> GSHMQDPEQLKHCNGILKELLSKKHAAYAWPFYKPVDASALGLHD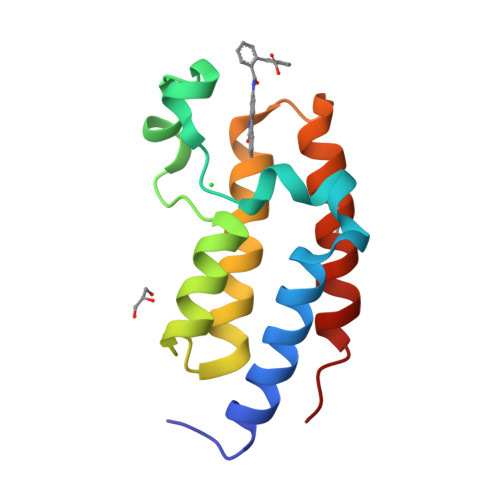YHDIIKHPMDLSTVKRKMENRDYRDAQEFAADVRLMFSNCYKYNPPDHDVVAMARKLQDVFEFRYAKMPA>MTWLPLNPIPLKDRVSMIFLQYGQIDVIDGAFVLIDKTGIRTHIPVGSVACIMLEPGTRVSHAAVRLAAQVGTLLVWVGEAGVRVYASGQPGGARSDKLLYQAKLALDEDLRLKVVRKMFELRFGEPAPARRSVEQLRGIEGSRVRATYALLAKQYGVTWNGRRYDPKDWEKGDTINQCISAATSCLYGVTEAAILAAGYAPAIGFVHTGKPLSFVYDIADIIKFDTVVPKAFEIARRNPGEPDREVRLACRDIFRSSKTLAKLIPLIEDVLAAGEIQPPAPPEDAQPVAIPLPVSLGDAGHRSS[4x];>[2x]MSMLVVVTENVPPRLRGRLAIWLLEVRAGVYVGDVSAKIR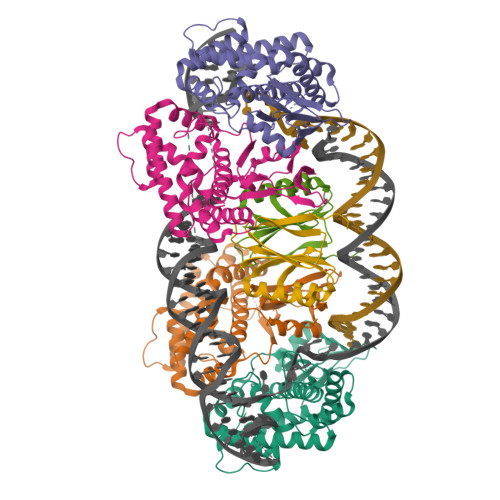EMIWEQIAGLAEEGNVVMAWATNTETGFEFQTFGLNRRTPVDLDGLRLVSFLPVG> IVGGRRARPHAWPFMVSLQLRGGHFCGATLIAPNFVMSAAHCVANVNVRAVRVVLGAHNLSRREPTRQVFAVQRIFEDGYDPVNLLNDIVILQLNGSATINANVQVAQLPAQGRRLGNGVQCLAMGWGLLGRNRGIASVLQELNVTVVTSLCRRSNVCTLVRGRQAGVCFGDSGSPLVCNGLIHGIASFVRGGCASGLYPDAFAPVAQFVNWID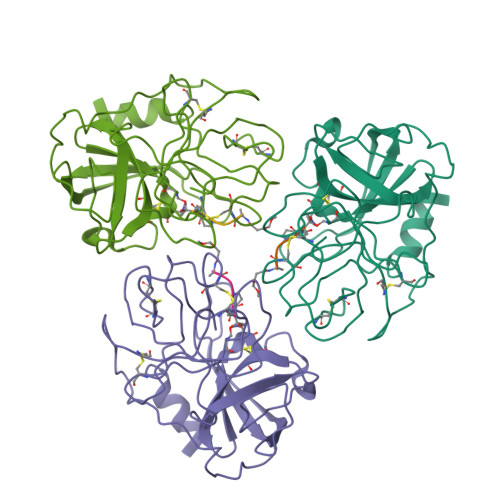SIIQ>[4x]AGSVDTVSLYSGRGANMPFTIMEAESTSNATNGTKLTPNFKPGDYAGEASGRSSVYLDATGEYVEFTLTSPANAFVLRNAVAENTTGTVSIYADGVSKGKFNVSSKFSYLYATPSTLGRLGYDNAPGAGLTAYWLYEDAQ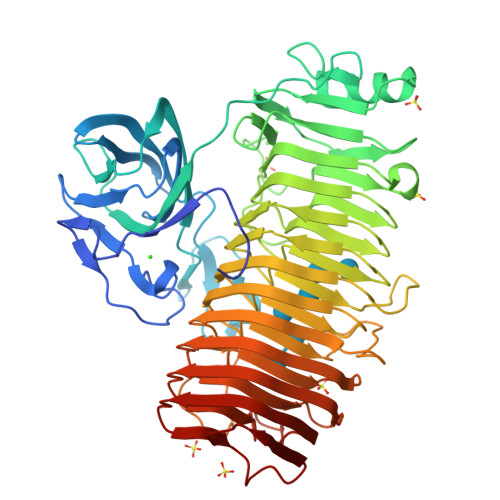LMLDQVYPAGTKIKIQKDAGDVSWIYVDLLETENVAPPQANPDPTKYVAVSASKSIDQALTEFRQDNTKKGIYIPAGEWTINSKIFLYGRATEIVGAGPWYTKLVAPQSQSNTDVGFNISAAANGSTIRDLSAWGNYINRVDGPGKFIDGNGMQNVTVQNIWVEHFVCLYWGVNSSYNTFKNNRIKNTFADGINMTNGSSYNVIDNNYARGTGDASFALFSATDSGGSYNVGNKYTNLTATNVRRAAAFAVYGGSDNLFQNLYGADTLTYPGITISSYSFGYNTLGFGDQDTVIDGATLDRTGGDFWTSVGADDKINEYQNFGAIWIYGGDRAIKNILIKNVDINNPVYFGLMFQSMSPNNMVMQNIRVENVNINNPSRYGIKLVVRAEQGQGPAYGGASFTNVKVNNPGISAIYGEAQSPNFTVTRVSGNNW>TPDRHQFPGLANKTYFNFGGQGILPTVALEAITAMYGYLQENGPFSIAANQHIQQLIAQLRQALAETFNVDPNTITITDNVTTGCDIVLWGLDWHQGDEILLTDCEHPGIIAIVQAIAARFGITYRFFPVAATLNQGDAAAVLANHLGPKTRLVILSHLLWNTGQVLPLAEIMAVCRRHQGNYPVRVLVDGAQSAGSLPLDFSRLEVDYYAFTGHAWFAGPAGVGGLYIHGDCLGEINPTYVGWRSITYGAKGEPTGWAEGGKRFEVATSAYPQYAGLLAALQLHQRQGTAEERYQAICQRSEFLWRGLNQLPHVHCLATSAPQAGLVSF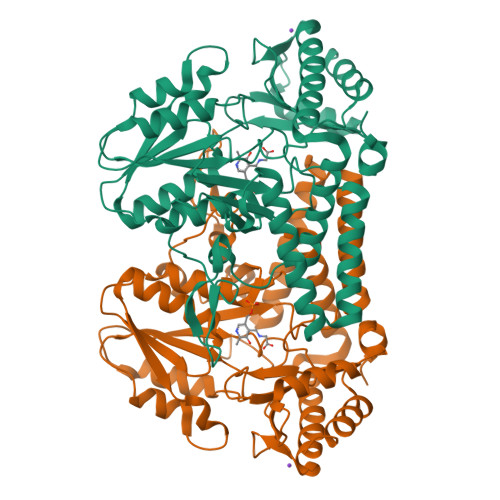TVDSPLGHRAIVQKLEEQRIYLRTIADPDCIRACCHYITDEEEINHLLARLADFGP[2x]> MDGRIKEVSVFTYHKKYNPDKHYIYVVRILREGQIEPSFVFRTFDEFQELHNKLSIIFPLWKLPGFPNRMVLGRTHIKDVAAKRKIELNSYLQSLMNASTDVAECDLVCTFFHGSHHHHHH

PX domains have specialized protein structures involved in binding of phosphoinositides (PIs). Through binding to the various PIs PX domains provide site-specific membrane signals to modulate the intracellular localisation and biological activity of effector proteins. While all PI3Ks must interact with phosphoinositides as phosphorylation substrates within the catalytic domain active site, membrane-associated class II PI3Ks are unique in that they additionally contain PX and C2 domains appended to the C-terminus of the kinase domain. The PI3K-C2α PX domain folds into the canonical PX polypeptide chain topology comprising a three-stranded β-sheet meander that packs against a subdomain of 3 α-helices.

The model obtained based on the 2.5 Å data contains coordinates for residues 1421–1532 of the domain and an additional GSHH tag-derived sequence at the C-terminus. Residues 1490, 1491 and 1493–1496 were modelled as alanines since their side-chains were not clearly visible in the electron-density maps. This model, which we refer to here as 'structure B', was refined to an Rfactor/Rfree of 0.231/0.311. Our two new structures, A and B, are however not identical: they have two significantly different conformations of the putative PI binding region. Our two new structures of PI3K-C2α PX domain show significantly different conformations of the PI binding region. These differences are attributed to the presence of a putative ligand in the PtdIns(4,5)P2 binding cavity in one of the crystal structures. The ligand-bound structure exhibits an 'open' conformation of the PI binding region. Structure B has a more open PI binding site with the PPII/α2 loop and β1-β2 turn presenting conformations similar to that previously seen in the yeast PX domain protein Grd19p. The closed conformation of structure A is more similar to the PtdIns3P-bound Grd19p structure, while the PI3K-C2α PX structure B is closer to the un-liganded Grd19p structure. In structure B, the putative ligand appears to form hydrogen bonds with Arg1503, a highly conserved residue in PX domains. Modelling of an inositol ring in this site shows that, with minor adjustments of torsion angles Arg1503 would be optimally posed to interact with a phosphoryl group at inositol position 4 and that another residue from PPII/α2 loop would likely be involved in interaction with the 5-phosphate.> MIVYNNQAPDAVNNVGQFGATEGSIGAYKQAAEYAADSKYWALLAESKFGTIDDLIAEVERLYQQGVLMKQDIEDLKQDFKDQDARLMSLIAQTNAAVSDANNAVALINQKLIEVQNQLDVLLGMSVDVTTLPPGTPATGSFNPNTGVISLGIPEGEPGKDGSVKDLDTAPTGVPELGDLGFYVDKDDNTVHKTTLENIANLTPSVRSVSVNGGPALDGEVALTINKETVGLGNVLNVAQYSRQEINDKFDKTTKTYQSKAEAYADAQYRQVGEKVLVWEATKYEFYTVAANKTLTPVKTEGRILTVNSRSPDSSGNIDITIPTGNPSLYLGEMVMFPYDPSKNISYPGVLPADGRLVSKESASDLGPSLVSGQLPVVSETEWQSGAKQYFSWGKLADGITDADSTNFINIRLPDWTGGEAIRAPDSDKDSQYNGSVQAQKPYVVTVNNQAPDEITGNVNISRSILGAASSGANSDITSLSGLTTPLSISQGGTGAKDAASARSNL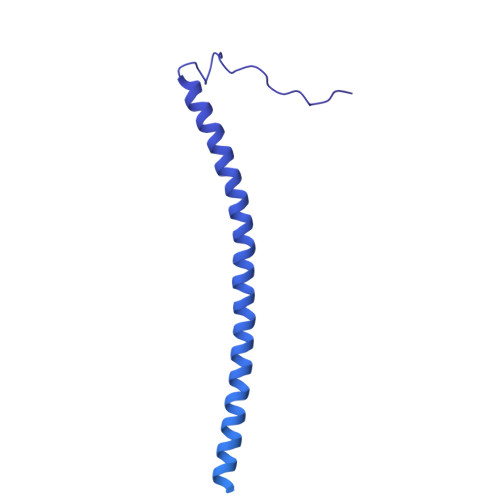GLGSVSTLDNVPIASGGTGAGDAAGARFNLGLGNSATMNTGTNSDNVLKVGDFGIGRPDGALVFDTTSQDQLLAGLDTYGLCVFRNNQQIAAPWDIWNYSSNLFFRAGDTYSMISIPFESAGKIKVFGGASGSGWKTSRTVYDTVNTTVDVNGFIKAASPIVKVFHDGSFETNEQSDGVSVKKISTGVYLISGCLGLNSDAGWGGVDGGFEIPIDRNKQPRVWLDYEVKEDGSLLIKTYHRTHSTSPAFARNELEGFSDGDPVDIPKDAFISVRVEMPSK> ASNLKIVRMDRTAGCVTGGEEIWLLCDKVQKDD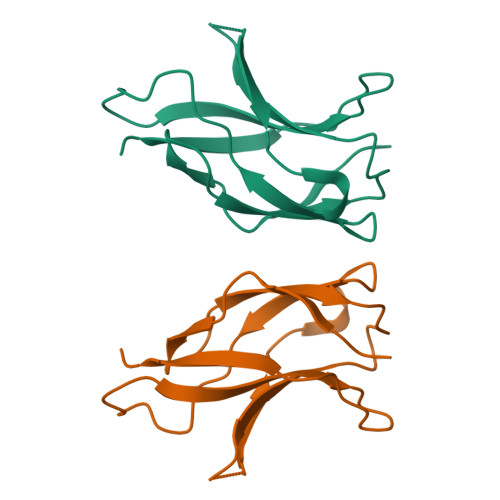IQIRFYEEEENGGVWEGFGDFSPTDVHRQFAICFKTPKYKDVNITKPASVFVQLRRKSDLETSEPKPFLYYPE> MAVSVGEGPDTKPTARGQPAAVGRVVVLSGPSAVGKSTVVRCLRERIPNLHFSVSATTRAPRPGEVDGVDYHFIDPTRFQQLIDQGELLEWAEIHGGLHRSGTLAQPVRAAAATGVPVLIEVDLAGARAIKKTMPEAVTVFLAPPSWQDLQARLIGRGTETADVIQRRLDTARIELAAQGDFDKVVVNRRLESACAELVSLLVGTAPGSPGVPRGKL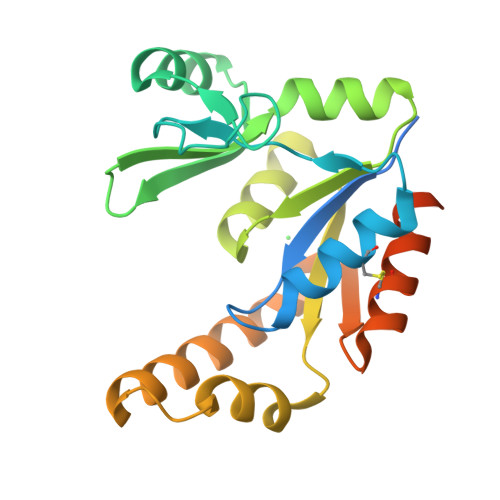AAALEHHHHHH> TEFKAGSAKKGATLFKTRCLQCHTVEKGGPHKVGPNLHGIFGAHSGQAEGYSYTDAIIKKNVLWDENNMSEYLTNPKKYIPGTKMAF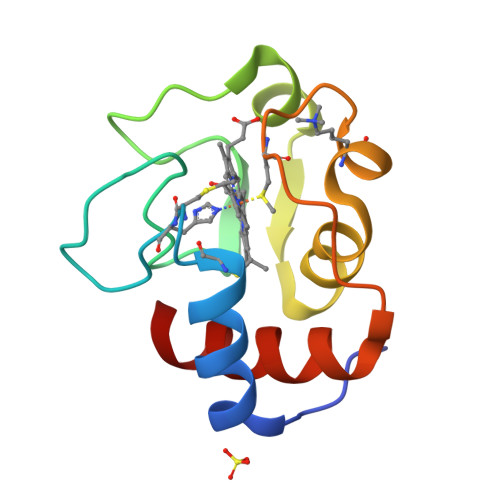GGLKKEKDRNDLITYLKKAAE Ngb is over-expressed in hypoxic conditions and it may be involved in gas/redox sensing, radical scavenging, and/or signal transduction. Notably, hexacoordination in Ngb accounts for a peculiar structural rearrangement and complex kinetics upon ligand binding, which takes place when the distal histidine (His(E7)64), engaged in internal iron hexacoordination, dissociates from the heme. The dissociation of His64 is the rate-limiting step for ligand binding and it triggers a repositioning of the heme which slides further inside a large internal cavity. In this study, we spectroscopically and structurally characterized three Ngb mutants aiming at pinpointing key features: a CD loop mutant with enhanced flexibility (Gly-loop), the F106A mutant and the double Gly-loop/F106A mutant.

Crystal structures of unliganded hexacoordinated F106A (1.8 Å) and carbomonoxy-F106A (F106A-CO, 1.75 Å), were determined to observe the effect of removal of the steric barrier to heme sliding posed by Phe106. At this resolution, we clearly detect the double heme conformation: the B conformer (canonical, 30% in ferric F106A, 27% in F106A-CO) and the A one (reversed, 70% in ferric F106A, 73% in F106A-CO). However, the most striking observation about heme conformations is the relative position of the A and B conformers, that are laterally and vertically shifted, with their iron atoms being about 1.0 Å and 0.90 Å apart, respectively in the unliganded and in the carbomonoxy form. In addition, the Fe-Fe distance between hexacoordinated F106A and F106A-CO shows, upon CO binding, a displacement of the heme A conformer of about 2.3 Å and of 2.9 Å for the heme B conformer, larger than the one observed for WT Ngb (2.0 Å15). The enhanced displacement of B conformer is due to the absence of Phe106 ring onto which the heme leans in the WT protein. In the F106A-CO structure, the absence of Phe in position 106, associated with the two heme insertion modes, induces residues such as Trp148 and the whole FG loop to explore multiple conformations upon heme sliding. This structural feature could account for the biphasic behaviour detected in CO binding. The evaluation of the fast and slow binding phases in CO mixing experiment allows us to attribute to the B conformer the slow binding fraction and to the A conformer the fast binding one. The effect of the double heme insertion observed in Ngb is enhanced by the increased size of the large Ngb internal cavity created by the F106A mutation, which results in a set of alternate conformations of proximal side residues that account for the enhanced biphasic behaviour in ligand binding of mutants carrying this substitution.

> MERPESELIRQSWRVVSRSPLEHGTVLFARLFALEPSLLPLFQYNGRQFSSPEDSLSSPEFLDHIRKVMLVIDAAVTNVEDLSSLEEYLTSLGRKHRAVGVRLSSASTVGESLLYMLEKSLGPDFTPATRTAWSRLYGAVVQAMSRGWDGE> MPSGLRGYNVYRNGVRQNTSPVTELGSVTITGLTPGTDYSSQITVTAIDMAGNESEPKTLAELEAEAATDELSPADPLAPAVRAQIDALVAAKMKPTSGKEADGAMVGIETPTGSYYKAYGGDRTKNQPLFLEQNFRYGSCSKMACNTLLLREIDRGHVDWDDTLDQFIDGIPNGDKITVRYLLLFQDGLKDWLQGDPAVQQTYFLNPTLNYDPLAYIRASTPVFEPGTDSHYSNAATLLMGKILEWCDAEFYTGRSARELIVEEWKNTVGMESLHWPTTNYMNQPYVRGWTPNMALPQIQAILGPFAFLAGLLGYPTSKDLEWTAVSTTWSDAAGSLAGNMEDFVKFGKALYEG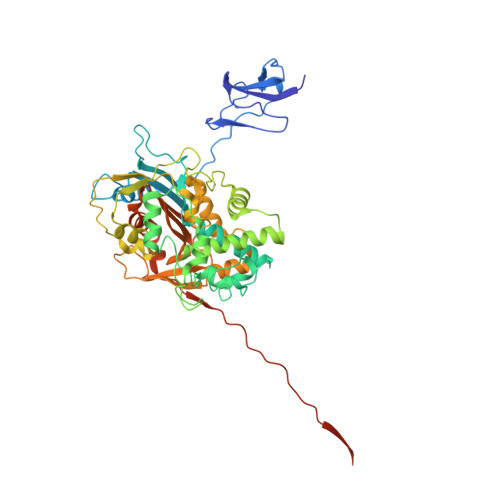EFLSEEMNQLRKEIFTRYVEYEPAGPHQGPGWMGFGLNSICWGHWLGWVGNLGGYIAVLFYNQDDGSVIATMLNNFAGHADAVDLFYQIAYLLNPESTGHRDWIFRPDPAEDADEVRDPTLYLTVESTGDNQIPADVPFEI>C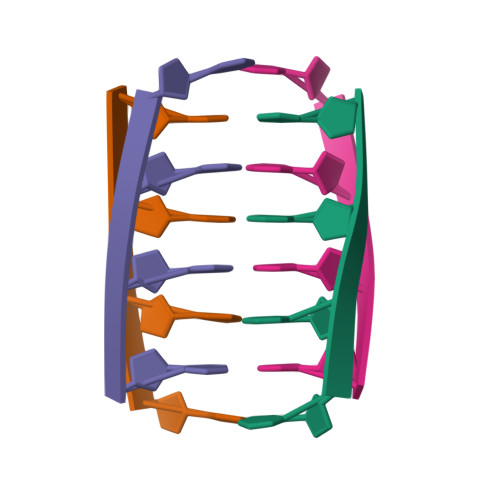CCC[8x]>GAARIMLLERTLQLKEEENKRLNQRLMSQSMSSVSSRHSEKIAIRDFQVGDLVLIILDERHDNYVLFTVSPTLYFLHSESLPALDLKPGEGASGASRRPWVLGKVMEKEYCQA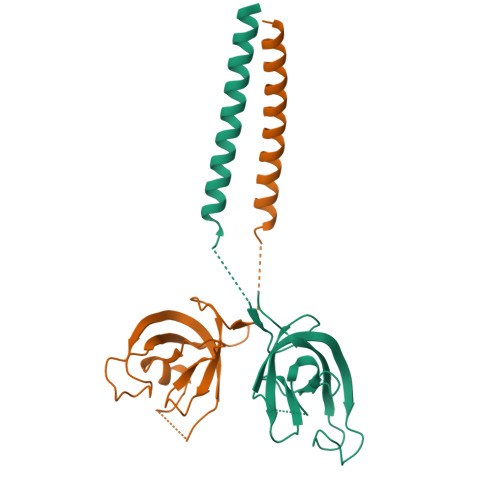KKAQNRFKVPLGTKFYRVKAVSWNKKV[6x]> MGFLSGKRILVTGVASKLSIAYGIAQAMHREGAELAFTYQNDKLKGRVEEFAAQLGSDIVLQCDVAEDASIDTMFAELGKVWPKFDGFVHSIGFAPGDQLDGDYVNAVTREGFKIAHDISSY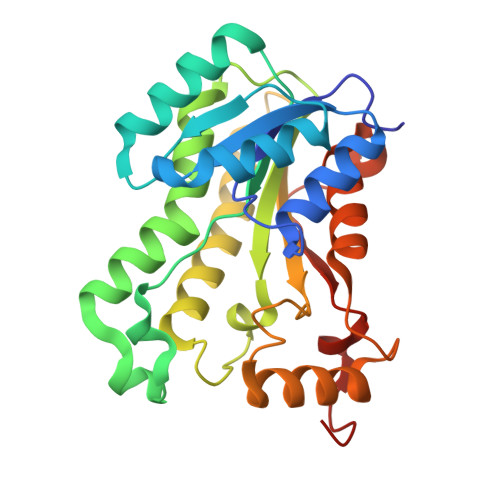SFVAMAKACRSMLNPGSALLTLSYLGAERAIPNYNVMGLAKASLEANVRYMANAMGPEGVRVNAISAGPIRTLAASGIKDFRKMLAHCEAVTPIRRTVTIEDVGNSAAFLCSDLSAGISGEVVHVDGGFSIAAMNELELK>KKKIVDANIATETMIDINVGGAIFETSRHTLTQQKDSFIEKLLSGRHHVTRDKQGRIFLDRDSELFRIILNFLRNPLTIPIPKDLSESEALLKEAEFYGIKFLPFPLVFCIGGFDGVEYLNSMELLDISQQCWRMCTPMSTKKAYFGSAVLNNFLYVFGGNNYDYKALFETEVYDRLRDVWYVSSNLNIPRRNNCGVTSNGRIYCIGGYDGSSIIPNVEAYDHRMKAWVEVAPLNTPRSSAMCVAFDNKIYVIGGTNGERLNSIEVYE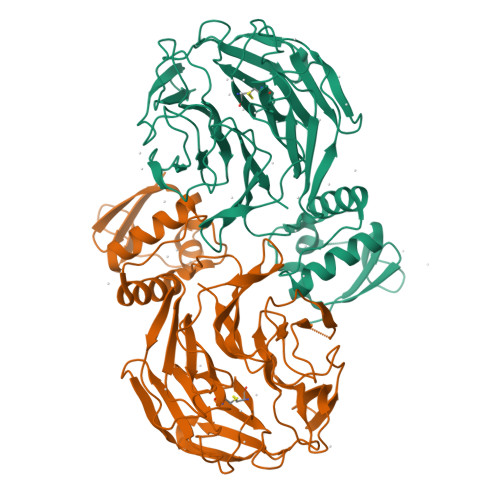EKMNKWEQFPYALLEARSSGAAFNYLNQIYVVGGIDNEHNILDSVEQYQPFNKRWQFLNGVPEKKMNFGAATLSDSYIITGGENGEVLNSCHFFSPDTNEWQLGPSLLVPRFGHSVLIANI[2x]CALYSTEGINE B2 | C7 H13 N O4 | 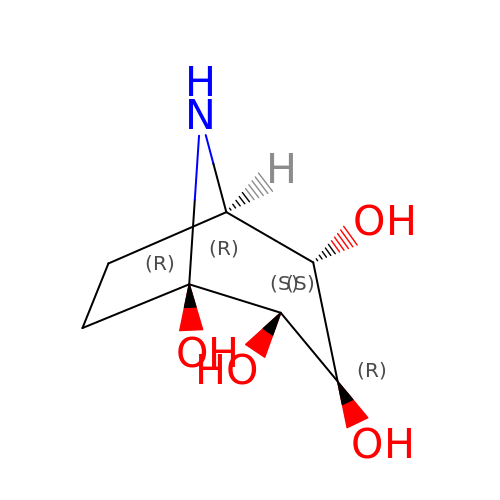FXFBVZOJVHCEDO-IBISWUOJSA-N> MASKTTSEELKTATALKKRSSDVHAVDHSGNVYKGFQIWTDLAPSVKEEPDLMFAKCIVQAGTDKGNLTCVQIDPPGFDEPFE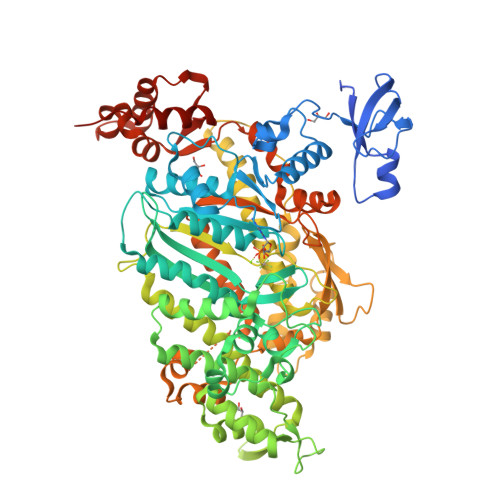VPQANAWNVNSLIDPMTYGDIGMLPHTNIPCVLDFLKVRFMKNQIYTTADPLVVAINPFRDLGNTTLDWIVRYRDTFDLSKLAPHVFYTARRALDNLHAVNKSQTIIVSGESGAGKTEATKQIMRYFAAAKTGSMDLRIQNAIMAANPVLEAFGNAKTIRNNNSSRFGRFMQLDVGREGGIKFGSVVAFLLEKSRVLTQDEQERSYHIFYQMCKGADAAMKERFHILPLSEYKYINPLCLDAPGIDDVAEFHEVCESFRSMNLTEDEVASVWSIVSGVLLLGNVEVTATKDGGIDDAAAIEGKNLEVFKKACGLLFLDAERIREELTVKVSYAGNQEIRGRWKQEDGDMLKSSLAKAMYDKLFMWIIAVLNRSIKPPGGFKIFMGMLDIFGFEVFKNNSLEQFFINITNEMLQKNFVDIVFDRESKLYRDEGVSSKELIFTSNAEVIKILTAKNNSVLAALEDQCLAPGGSDEKFLSTCKNALKGTTKFKPAKVSPNINFLISHTVGDIQYNAEGFLFKNKDVLRAEIMEIVQQSKNPVVAQLFAGIVMEKGKMAKGQLIGSQFLSQLQSLMELINSTEPHFIRCIKPNDTKKPLDWVPSKMLIQLHALSVLEALQLRQLGYSYRRPFKEFLFQFKFIDLSASENPNLDPKEAALRLLKSSKLPSEEYQLGKTMVFLKQTGAKELTQIQRECLSSAAAENLYFQ Lyn kinase (Lck/Yes related novel protein tyrosine kinase) is a Src-family kinase organized into four domains. These include an N-terminal unique domain (also known as SH4 domain), two adapter domains (SH3 and SH2) and C-terminal kinase domain (also known as SH1 domain). In the inactive state, the SH3 domain binds to the linker between the SH2 domain and the kinase domain, keeping the kinase in a closed (inactive) conformation. SH2 and SH3 adapter domains regulate the interactions of Lyn kinase with substrates and may help confer substrate specificity.

Here, we determined the structure of the Lyn SH3 domain to 1.3 Å resolution using X-ray crystallography, which allowed up to propose how cancer-associated point mutations affect this domain. The crystal structure of the Lyn SH3 domain contains five β-strands organized into two β-sheets. Previously termed β1 –β5, these β-strands are connected via four loops termed the RT loop, n-src loop, distal loop, and 310 helical loop. The largest differences in position involve the residues that are found within the polyproline binding cleft, G76, H78 and P79 of the RT loop and E98, E99 of n-src loop, which exhibit positional differences of 1.5 Å – 2.3 Å due to rotation of these loop elements. Conformational changes in these two loops are observed in the NMR structure bound to the herpesvirus-derived peptide. Flexibility of the RT and n-src loops has previously been suggested as important for interaction with polyproline motifs, which might proceed via an induced fit mechanism. Analysis of whole genomes revealed 18 cancer-associated point mutations within the Lyn SH3 domain, affecting ~30% of the residues in this domain. Evaluation of the locations of these mutations in the context of the structure suggests that many of the likely transformative substitutions could prevent the interaction of the SH3 domain with the kinase domain, but by distinct mechanisms. For example, a subset of the mutations, including D81N, W99L and E98K, may disrupt the protein-protein interaction interface with the kinase domain, and eliminate negative regulation of kinase activity. Other mutations, such as V118M, may destabilize the fold of the SH3 domain, again preventing the normal attenuation of kinase activity in the basal state of Lyn.

> EQGDIVVALYPYDGIHPDDLSFKKGEKMKVLEEHGEWWKAKSLLTKKEGFIPSNYVAKLNTLEHHHHHH>FDCGKPQVEPKKCPGRVVGGCVAHPHSWPWQVSLRTRFGMHFCGGTLISPEWVLTAAHCLEKSPRPSSYKVILGAHQEVNLEPHVQEIEVSRLFLEPTRKDIALLKLSSPAVITDKVIPACLPSPNYVVADRTECFITGWGETQGTFGAGLLKEAQLPVIENKVCNRYEFLNGRVQSTELCAGHLAGGTDSCQGDSGGPLVCFEKDKYILQGVTSWGLGCARPNK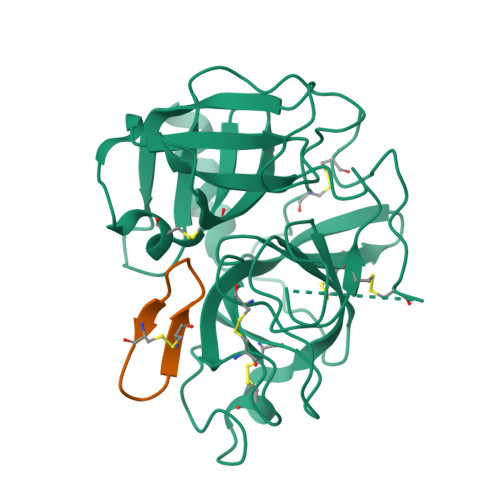PGVYVRVSRFVTWIEGVMRNN[2x];>GRCYKSKPPICFPD[2x]3'-O-ACETYLTHYMIDINE-(5' DIPHOSPHATE PHENYL ESTER) | C18 H22 N2 O12 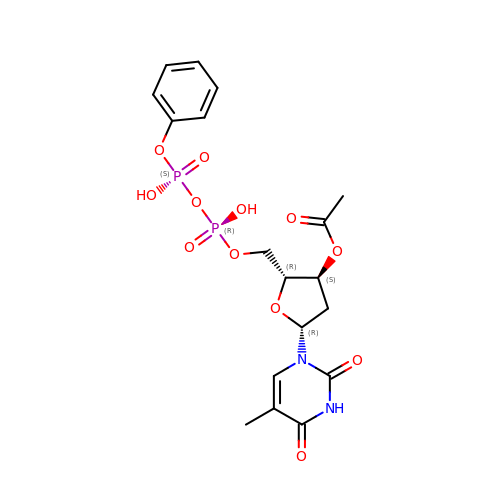P2 | FBXZTUIVKSOQAY-ARFHVFGLSA-N> MAHHHHHHMLKAEIFSGVIPALMTPCKPDRSPDFDALVRKGQELIGDGMSAVVYCGSMGDW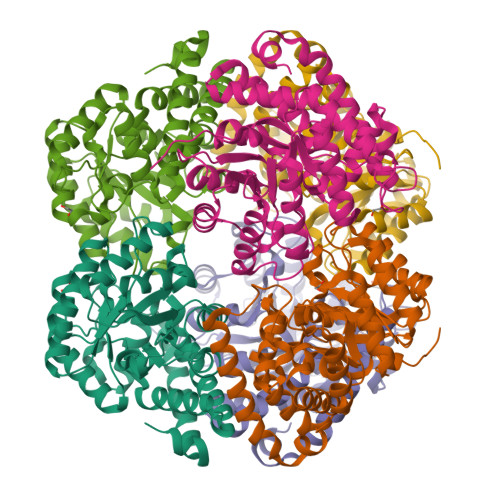PLLTDAQRMEGVERLVKAGIPVIVGTGAVNTASAVAHAAHAQKVGAKGLMVIPRVLSRGSAIAAQKAYFKAILSAAPDLPAVIYNSPYYGFATRADLFFDLRAEHPNLVGFKEFGGPADMRYAAENITSRDDGVSLMIGVDTAVFHGFVNCGATGAITGIGNVLPKEVIHLCNLSQAAALGDVDARQRAQELEQALAVLSSFDEGPDLVLYFKHMMVLKGDKEYTLHFNETDALSESQRGYVETQFRLFNTWYAEWSKLPGAVQRCKA> CCG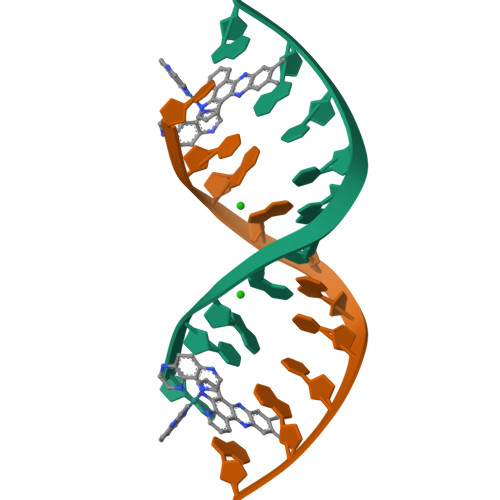GCGCCGG>GASARLLRAAIMGAPGSGKGTVSSRITKHFELKHLSSGDLLRDNMLRGTEIGVLAKTFIDQGKLIPDDVMTRLVLHELKNLTQYNWLLDGFPRTLPQAEALDRAYQIDTVINLNVPFEVIKQRLTARWIHPGSGRVYNIEFNPPKTMGIDDLTGEPLVQREDDRPETVVKRLKAYEAQT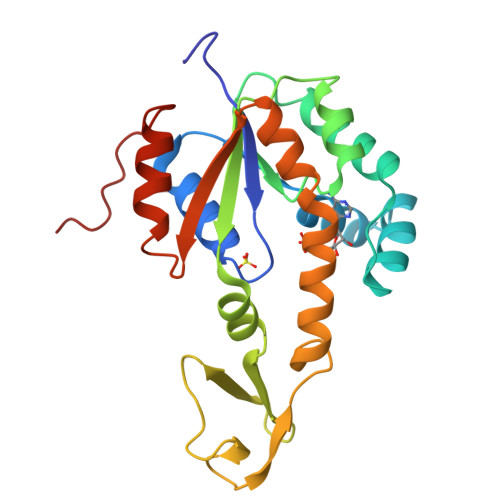EPVLEYYRKKGVLETFSGTETNKIWPHVYAFLQTKLPQRSQETSVTP[2x]> MNGWNFQELKETPSQTGGPYVHIGLLPKQANIEVFEHNLDNNLVQDNTQGQRIRLEGQVFDGLGLPLRDVLIEIWQADTNGVYPSQA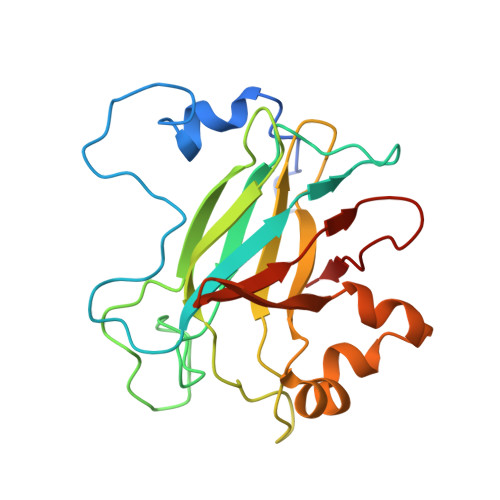DTQGKQVDPNFLGWGRTGADFGTGFWSFNTIKPGAVPGRKGSTQAPHISLIIFARGINIGLHTRVYFDDEAEANAKDPVLNSIEWATRRQTLVAKREERDGEVVYRFDIRIQGENETVFFDI>GSHMASTTPLPLEPIETASRDELTALQLERLKWSLRHAYDHSPVYRRKFDEAGVHPDDLKTLADLSRFPFTTKGDLRDSYPFGMFAVPQDRISRIHASSGTTGKPTVVGYTAADIDTWANLVARSIRAAGARRGDKVHVSYGYGLFTGGLGAHYGAERAGLTVIPFGGGQTEKQVQLIQDFRPDIIMVTPSYMLSIADEIERQGLDPVQSSLRIGIFGAEPWTNDMRVAIEQRMGIDAVDIYGLSEVMGPGVASECVETKDGPTIWEDHFY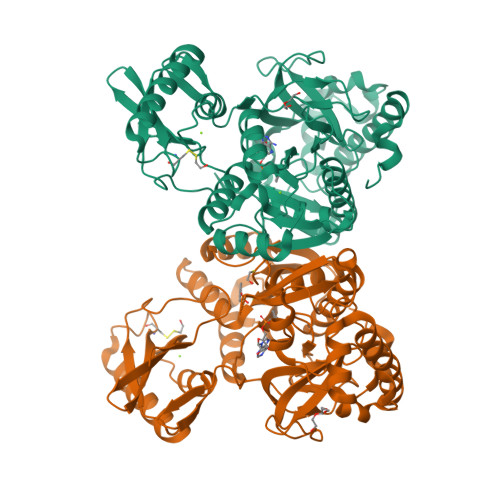PEIIDPETGEVLPDGELGELVFTSLTKEALPIIRYRTRDLTRLLPGTARTMRRMEKITGRSDDMMIVRGVNVFPTQIEEQLLKQRALAPHYQIVLTKEGPLDVLTLNVEPCPETAPDTAAIQVAKQALAYDIKSLIGVTAVINVLPVNGIERSVGKARRVVDKRKG[2x]> MRITTKVGDKGSTRLFGGEEVWKDDPIIEANGTLDELTS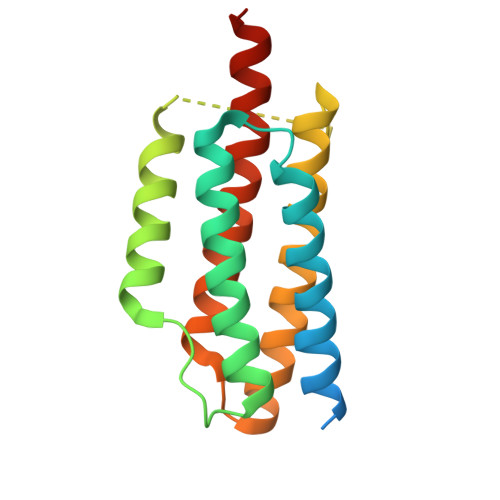FIGEAKHYVDEEMKGILEEIQNDIYKIMGEIGSKGKIEGISEERIKWLAGLIERYSEMVNKLSFVLPGGTLESAKLDVCRTIARRAERKVATVLREFGIGTLAAIYLALLSRLLFLLARVIEIEKNKLKEVRS> ISIGYLLVKHSQTDQEPMCPVGMNKLWSGYSLLYFEGQEKAHNQDLGLAGSCLARFSTMPFLYCNPGDVCYYASRNDKSYWLSTTAPLPMMPVAEEDIRPYI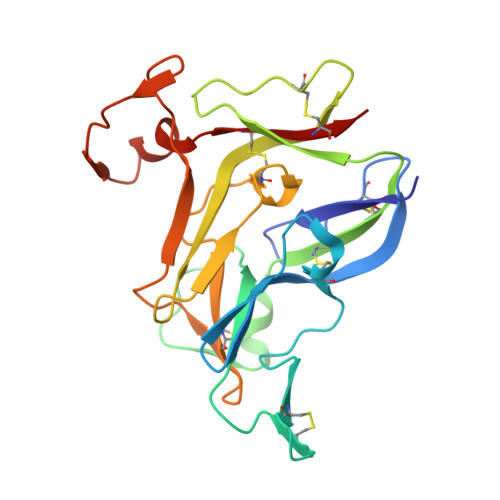SRCSVCEAPAVAIAVHSQDVSIPHCPAGWRSLWIGYSFLMHTAAGDEGGGQSLVSPGSCLEDFRATPFIECNGARGTCHYYANKYSFWLTTIPEQSFQGTPSADTLKAGLIRTHISRCQVCMKNL(2S)-2-(7-amino-4,5-dioxo-1,4,5,6-tetrahydropyrimido[4,5-c]pyridazin-3-yl)propanoic acid | C9 H9 N5 O4 | 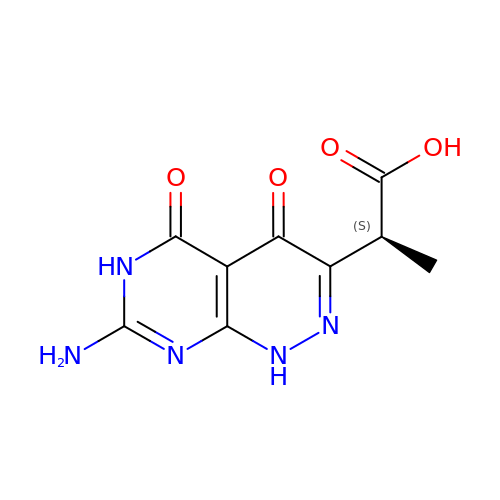GMTZUGVMBRNPHI-REOHCLBHSA-N hydrolysed ertapenem | C22 H27 N3 O8 S | 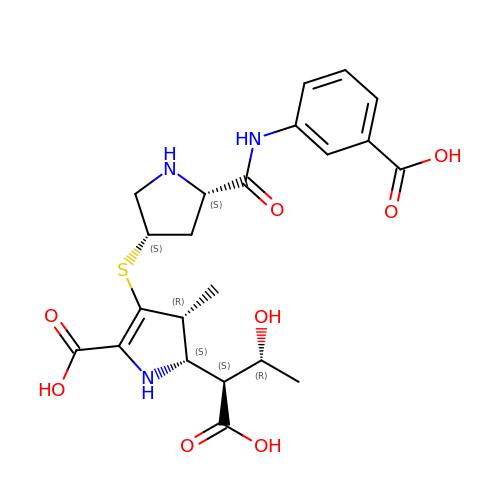LMDXYCKWMWUYCV-ANEDZVCMSA-N With the exception of a subset of lipoproteins that carry a transport avoidance signature and remain in the inner membrane, the majority of lipoproteins are destined for the outer membrane. Their transport is directed by the Lol system that comprises the inner membrane transporter LolCDE, the periplasmic chaperone LolA, and the outer membrane receptor LolB, itself a lipoprotein. Following maturation on the inner membrane and extraction by the LolCDE transporter, lipoproteins are passed to the chaperone LolA that carries them across the periplasm prior to insertion into the outer membrane by the LolB receptor. LolA and LolB share structural homology, both being incomplete β-barrels with a central hydrophobic cavity closed by an alpha helical lid, but perform distinct functions. Here, we present the crystal structure of LolA in complex with a lipoprotein, providing a molecular description of the interaction and a rationale for the capacity of the chaperone protein to transport evolutionarily divergent lipoproteins.

The importance of R43 in the lipoprotein transfer process was underlined by the identification of a mutant at this position, R43L, that though competent to accept lipoproteins from LolCDE was unable to transfer them to LolB. To resolve these possibilities, we produced the LolA R43L–lipoprotein complex and determined its crystal structure. The protein conformation is similar to that of liganded WT LolA with an rmsd of 0.68 Å over 167 residues, but the three acyl chains of Pal are positioned differently in the protein cavity. Here, the R1 and R3 chains run almost parallel with R2 inserting in the middle at the cavity base. The R1 chain is less deeply inserted in the R43L protein cavity by about 4 Å compared to its position in the wild-type structure. The cysteine carbonyl is rotated by about 180°, pointing toward the β-barrel curve in the R43L complex while facing the helical lid in the wild-type LolA structure. First, the F140 side chain is flipped toward the β-barrel curve of the protein, in a position that conflicts with the location of chain R1 observed in the wild-type complex structure. Second, the shallower insertion of the ligand means that Y152 is unable to interact with the R2 acyl chain carbonyl as it does in the wild-type structure. Instead, E144 situated nearer the mouth of the cavity forms a hydrogen bond with the carbonyl backbone of acyl chain R1. We found that the Pal +1 cysteine observed in the LolA R43L structure sterically clashes with LolB, while in the LolA wild-type structure, it is accommodated in a LolA surface groove allowing the linker joining the triacyl group to the lipoprotein mature domain to exit the complex.

> DAASDLKSRLDKVSSFHASFTQKVTDGSGAAVQEGQGDLWVKLPNLFNWHMTQPDESILVSDGKTLWFYNPFVEQATATWLKDATGNTPFMLIARNQSSDWQQYNIKQNGDDFVLTPKASNGNLKQFTINVGRDGTIHQFSAVEQDDQRSSYQLKSQQNGAVDAAKFTFTPPQGVTVDDQRKGSWSHPQFEK> MGERPPPKRLTREAMRNYLKERGDQTVLILHAKVAQKSYGNEKRFFCPPPCVYLMGSGWKKKKEQMERDGCSEQESQPCAFIGIGNSDQEMQQLNLEGKNYCTAKTLYISDSDKRKHFMLSVKMFYGNSDDIGVFLSKRIKVISKPSKKKQSLKNADLCIASGTKVALFNRLRSQTVSTRYLHVEGGNFHASSQQWGAFFIHLLDDDESEGEEFTVRDGYIHYGQTVKLVCSVTGMALPRLIIRKVDKQTALLDADDPVSQLHKCAFYLKDTERMYLCLSQERIIQFQATPCPKEPNKEMINDGASWTIISTDKAEYTFYEGMGPVLAPVTPVPVVESLQLNGGGDVAMLELTGQNFTPNLRVWFGDVEAETMYRCGE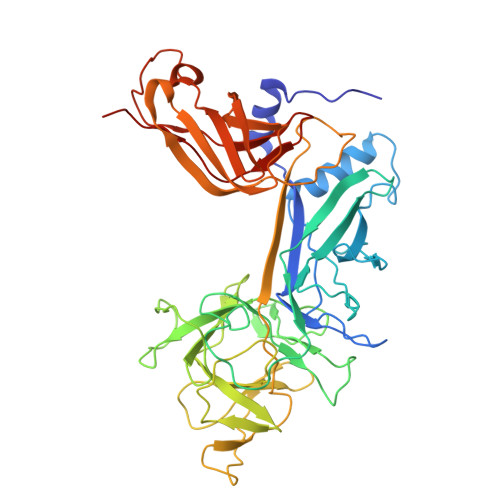SMLCVVPDISAFREGWRWVRQPVQVPVTLVRNDGIIYSTSLTFTYTPEPGHHHHHH> GSTGSDNQYKFKLKNITDSVEQALKIAKQIKDDLDIIEFHRIKLSNHYGIRAEEHEKQTAREELSKFSKDKLEADLKKLLSEIEKSLNAATILITYNDYGGNLQSDLSAKTTLEALKTEVSSLITKIQDFNNKDHQAYPTSYYNDYQTYQALRNPYSKLTLVKDLLTRT

B. miyamotoi encodes two separate bbk32 orthologs denoted fbpA and fbpB; however, the activities of these proteins are unknown. FbpA and FbpB both bind human complement C1r and protect a serum-sensitive B. burgdorferi strain from complement-mediated killing, but surprisingly, differ in their ability to recognize activated C1r versus zymogen states of C1r. To better understand the observed differences in C1r recognition and inhibition properties, high-resolution X-ray crystallography structures were solved of the C1r-binding regions of B. miyamotoi FbpA and FbpB at 1.9Å and 2.1Å, respectively. The crystal structures presented here of FbpA-C and FbpB-C show that a defining feature of the C1r-binding domains for BBK32 and B. miyamotoi Fbps is a four-helix core with an extended second alpha helix that presents a functional arginine residue on a small surface-loop.

A structural overlay of FbpA-C, FbpB-Δ5C, and BBK32-C shows that the three proteins retain an overall similar structure around the conserved R248 residue (BBK32 numbering). However, we noted that the area near BBK32-K327 involves a minor structural alteration in FbpA-C and a more major alteration in FbpB-Δ5C. More strikingly, the structure of FbpB-Δ5C has a significantly altered secondary structure in this region when compared to both FbpA-C and BBK32-C. Specifically, FbpB-Δ5C shows a loss of secondary structure within alpha helix 5 that accommodates a loop insertion sequence (i.e., residues Q394-Q405), which are not conserved in both BBK32-C or FbpA-C. Furthermore, a proline residue (P397) in this sequence interrupts the alpha helical secondary structure in FbpB-Δ5C. A portion of this unique loop structure in FbpB has apparent increased disorder in the crystal structure, indicated by weak electron density surrounding residues 401-403 in this region of the protein. We have previously shown that residues on the fifth alpha helix of BBK32 interact with a non-active site loop on C1r known as the B-loop. Interestingly, although BBK32-K327 is not conserved in FbpB, this did not preclude high-affinity interaction with activated C1r-CCP2-SP. FbpB-C blocked complement activation but, surprisingly, was ~80-fold less potent than FbpA (IC50 = 1,900 nM) despite having similar high affinity for activated C1r-CCP2-SP. Unlike BBK32/FbpA, FbpB fails to interact with zymogen forms of human C1r but instead selectively binds and inhibits the activated form. However, in our serum sensitivity assays, where B. miyamotoi FbpA and FbpB were produced ectopically on the surface of B. burgdorferi, both proteins conferred significantly greater protection to B314 than FbpA DA or the vector-only control. These data suggest that within the physiological context of complement activation on the spirochete surface, FbpB’s inhibition of activated C1r is sufficient to prevent downstream complement activation.> DITVYNGQHKEAATAVAKAFEQETGIKVTLNSGKSEQLAGQLKEEGDKTPADVFYTEQTATFADLSEAGLLAPISEQTIQQTAQKGVPLAPKKDWIALSGRSRVVVYDHTKLSEKD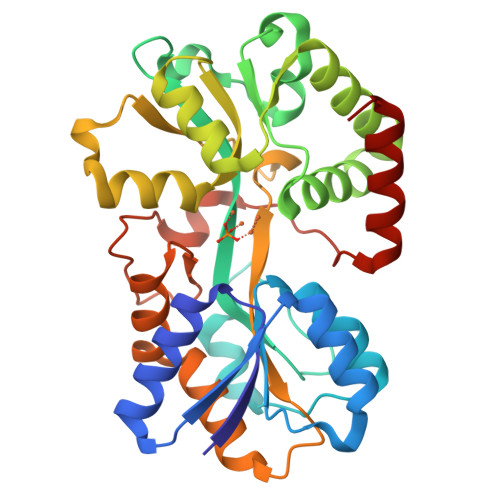MEKSVLDYATPKWKGKIGYVSTSGAFLEQVVALSKMKGDKVALNWLKGLKENGKLYAKLSVALQAVENGEVPAALINNYYWYNLAKEKGVENLKSRLYFVRHQDPGALVSYSGAAVLKASKNQAEAQKFVDFLASKKGQEALVAARAEYPLRADVVSPFNLEPYEKLEAPVVSATTAQDKEHAIKLIEEAGLK> PEARAELSSRLTTLRNTLAPATNDPRYLQACGGEKLNRFRDIQCRRQTAVRADLNANYIQVGNTRTIACQYPLQSQLESHFRMLAENRTPVLAVLASSSEIANQRFGMPDYFRQ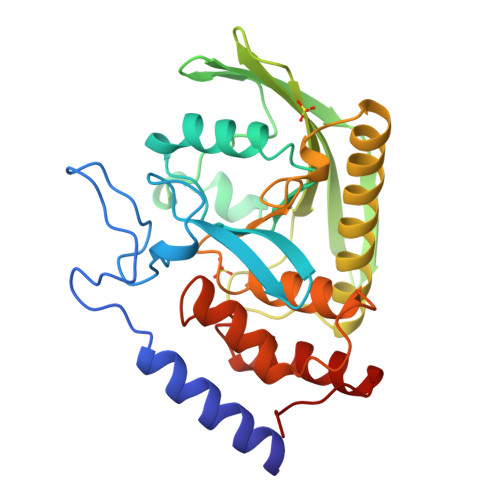SGTYGSITVESKMTQQVGLGDGIMADMYTLTIREAGQKTISVPVVHVGNWPDQTAVSSEVTKALASLVDQTAETKRNMYESKGSSAVADDSKLRPVIHSRAGVGRTAQLIGAMCMNDSRNSQLSVEDMVSQMRVQRNGIMVQKDEQLDVLIKLAEGQGRPLLNS> MAVAKATAAQRQEFLRQLNILAKDMY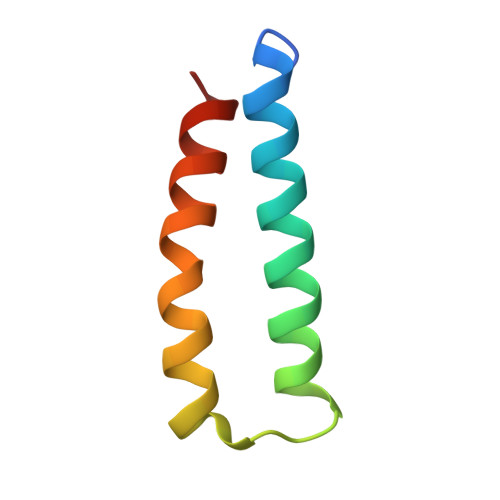QALTQPQDLAYRGPEIDAKIAALEAATAAVKAAS> QDFAEIYARFSDERANEQANRCSQCGVPFCQVHCPVSNNIPDWLKLTSEGRLEEAYEVSQATNNFPEICGRICPQDRLCEGNCVIEQSTHGAVTIGSVEKYINDTAWDQGWVKPRTPSRELGLSVGVIGAGPAGLAAAEELRAKGYEVHVYDRYDRMGGLLVYGIPGFKLEKSVVERRVKLLADAGVIYHPNFEVGRDASLPELRRKHVAVLVATGVYKARDIKAPGSGLGNIVAALDYLTTSNKVSLGDTVEAYENGSLNAAGKHVVVLGGGDTAMDCVRTAIRQGATSVKCLYRRDRKNMPGSQREVAHAEEEGVEFIWQAAPEGFTGDTVVTGVRAVRIHLGVADATGRQTPQVIEGSEFTVQADLVIKALGFEPEDLPNAFDEPELKVT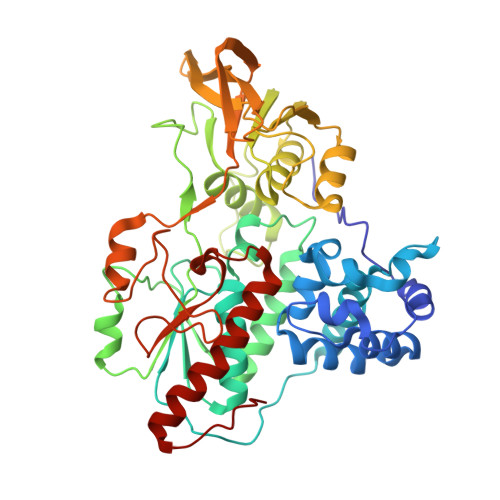RWGTLLVDHRTKMTNMDGVFAAGDIVRGASLVVWAIRDGRDAAEGIHAYAKAKAEAPVAVAAE>MDSFNPTTKTQAALTAALQAASTAGNPEIRPAHLLMALLTQNDGIAAPLLEAVGVEPATVRAETQRLLDRLPQATGASTQPQLSRESLAAITTAQQLATELDDEYVSTEHVMVGLATGDSDVAKLLTGHGASPQALREAFVKVRGSARVTSPEPEATYQALQKYSTDLTARAREGKLDPVIGRDNEIRRVVQVLSRRTKNNPVLIGEPGVGKTAIVEGLAQRIVAGDVPESLRDKTIVALDLGSMVAGSKYRGEFEERLKAVLDDIKNSAGQIITFIDELHTIVGAGATGEGAMDAGNMIKPMLARGELRLVGATTLDEYRKHIEKDAALERRFQQVYVGEPSVEDTIGILRGLKDRYEVHHGVRITDSALVAAATLSDRYITARFLPDKAIDLVDEAASRLRMEIDSRPVEIDEVERLVRRLEIEEMALSKEEDEASAERLAKLRSELADQKEKLAELTTRWQNEKNAIEIVRDLKEQLEALRGESERAERDGDLAKAAELRYGRIPEVEKKLDAALPQAQAREQVMLKEEVGPDDIADVV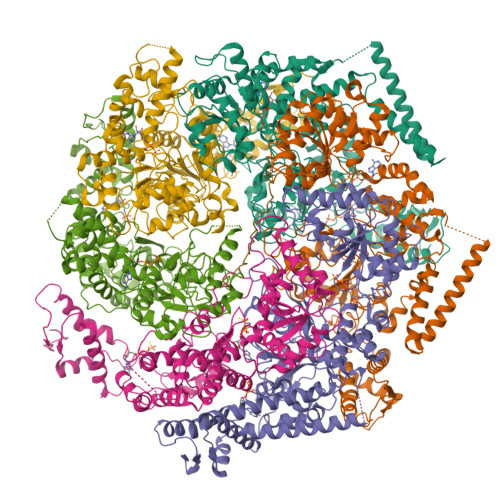SAWTGIPAGRLLEGETAKLLRMEDELGKRVIGQKAAVTAVSDAVRRSRAGVSDPNRPTGAFMFLGPTGVGKTELAKALADFLFDDERAMVRIDMSEYGEKHTVARLIGAPPGYVGYEAGGQLTEAVRRRPYTVVLFDEIEKAHPDVFDVLLQVLDEGRLTDGHGRTVDFRNTILILTSNLGSGGSAEQVLAAVRATFKPEFINRLDDVLIFEGLNPEELVRIVDIQLAQLGKRLAQRRLQLQVSLPAKRWLAQRGFDPVYGARPLRRLVQQAIGDQLAKMLLAGQVHDGDTVPVNVSPDADSLILG[6x];> AAAAAAAAAAAAAAAAAAAAAAAAAA5-bromo-1H-indazol-3-amine | C7 H6 Br N3 | 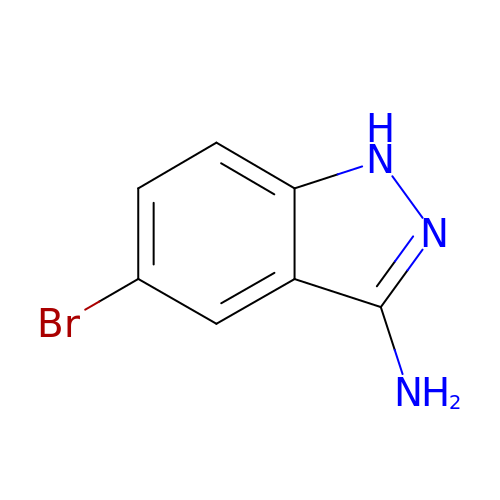OMPYFDJVSAMSMA-UHFFFAOYSA-N>MPTYKLTYFNFAGLGEPIRWMLSYLDVPFEDNRIEREQWPTIKSTTPYGQVPVLEVDGKQVCQSTAIARYLGKKAGLAGSNEWEDLMIDTMIDTFNDFRSSISKWFRESDEATKKKLEETLLNETVPFYFNKFNDHIKNNGGYLANGKLSWGDI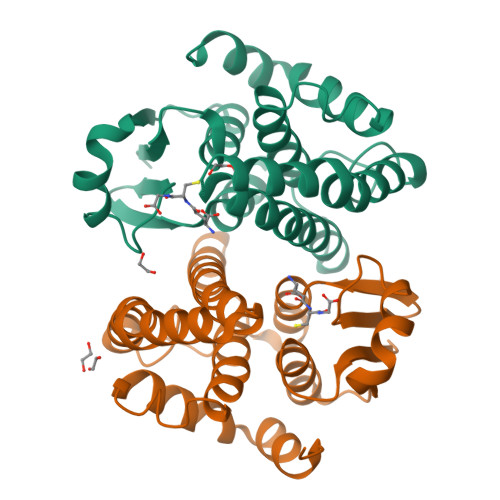YFISILEFMTTIWSDIIDKYEHIKALNDKVVNLPKIKAWIEKRPVPKK[2x]>[2x]MRIVFDIGGSVLVPENPDIDFIKEIAYQLTKVSEDHEVAVVVGGGK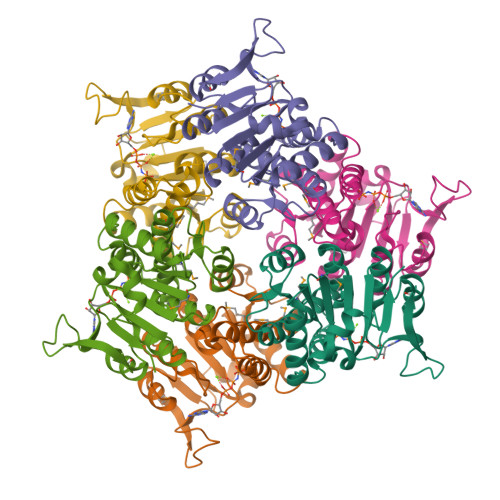LARKYIEVAEKFNSSETFKDFIGIQITRANAMLLIAALREKAYPVVVEDFWEAWKAVQLKKIPVMGGTHPGHTTDAVAALLAEFLKADLLVVITNVDGVYTADPKKDPTAKKIKKMKPEELLEIVGKGIEKAGSSSVIDPLAAKIIARSGIKTIVIGKEDAKDLFRVIKGDHNGTTIEP>[3x]MAKDPRYVGNLPKIGIRPTIDGRRKGVRESLEETTMNMAKAVAKLLEENVFYYNGQPVECVIADTCIGGVKEAAEAAEKFAREGVGVSITVTPCWCYGTETMDMDPHIPKAVWGFNGTERPGAVYLAAVLAGYNQKGLPAFGIYGKDVQDAGDTNIPEDVKEKLIRFAKAGLAVAMMKGKSYLSIGSVSMGIAGSVVQEDFFQNYLGMRNEYVDMSEFVRRIELGIYDKEEYERALKWVKENCKVGPDNNRDGFKRTEEQKEKDWEISVKMALIARDLMVGNKKLEEMGYGEEALGRNAIVAGFQGQRQWTDYFPNGDFMETILNSSFDWNGKRAPYIFATENDNLNGISMLFGYLLTNTAQIFADVRTYWSPEAVKRVTGYTLEGRAANGIIHLINSGAAALDGTGEQTKDGKPVIKPYYELTDEDIKKCLEATQFRPASTEYFRGGGYSTDFLTKGGMPVTISRLNIVKGLGPVLQIAEGYTVDLPEEVHDVLDKRT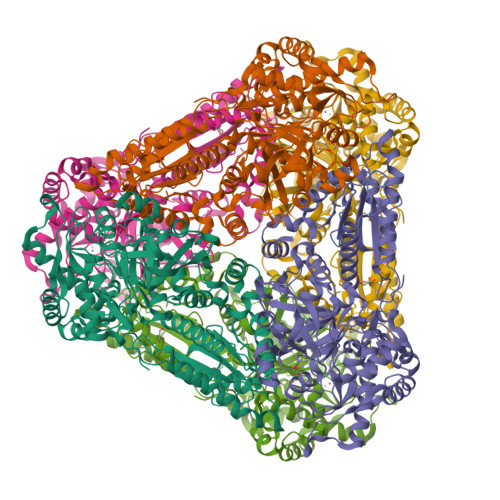DPTWPTTWFVPNLTGEGAFKDVYSVMNNWGANHCSISYGHIGADLITLASILRIPVNMHNVPEEKIFRPDAWSMFGTKDLEGADYRACKKLGPIYK> MVPELKQISRVEAMRLGPGWSHSCHAMLYAANPGQLFGRIPMRFSVLMQMRFDGLLGFPGGFVDRRFWSLEDGLNRVLGLGLGCLRLTEADYLSSHLTEGPHRVVAHL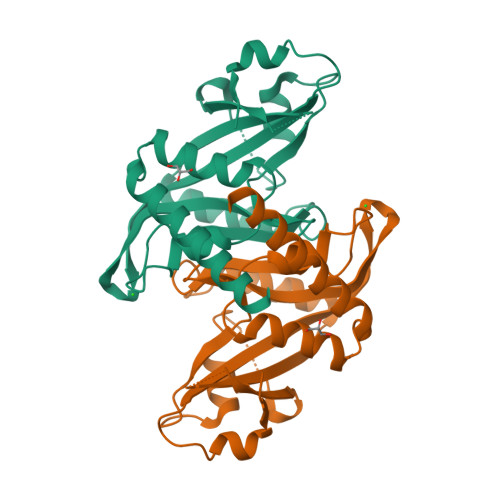YARQLTLEQLHAVEISAVHSRDHGLEVLGLVRVPLYTQKDRVGGFPNFLSNAFVSTAKCQLLFALKVLNMMPEEKLVEALAAATEKQKKALEKLLPASSAHHHHHH>[2x]MTTKQICFADRCFNFAFGEHVLESVESYIPRDEFDQYIMISDSGVPDSIVHYAAEY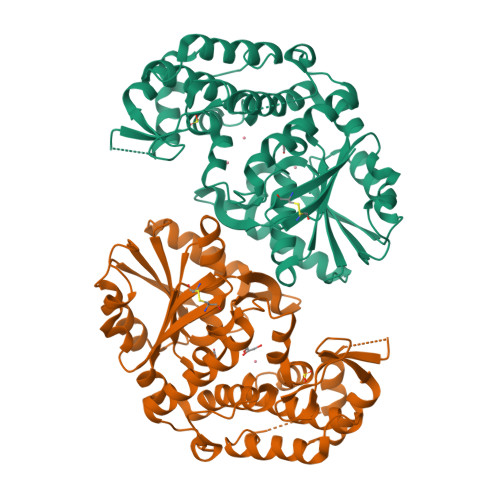FGKLAPVHILRFQGGEEYKTLSTVTNLQERAIALGANRRTAIVAVGGGLTGNVAGVAAGMMFRGIALIHVPTTFLAASDSVLSIKQAVNLTSGKNLVGFYYPPRFVFADTRILSESPPRQVKAGMCELVKNMLILENDNKEFTEDDLNSANVYSPKQLETFINFCISAKMSVLSEDIYEKKKGLIFEYGHTIGHAIELAEQGGITHGEAIAVGMIYAAKIANRMNLMPEHDVSAHYWLLNKIGALQDIPLKSDPDSIFHYLIHDNKRGYIKLDEDNLGMILLSGVGKPAMYNQTLLTPVRKTLIKEVIREGL>MMSETAPLPSASSALEDKAASAPVVGIIMGSQSDFETMRHADALLTELEIPHET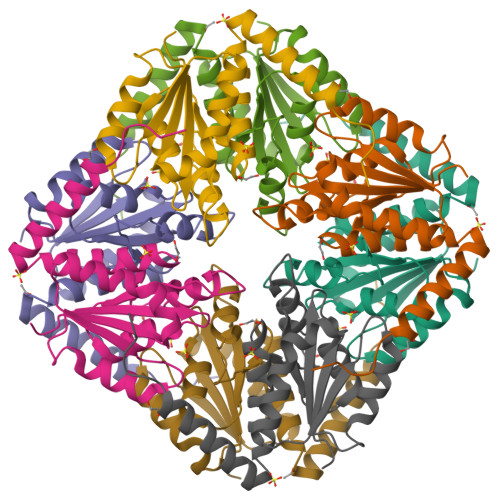LIVSAHRTPDRLADYARTAAERGLNVIIAGAGGAAHLPGMCAAWTRLPVLGVPVESRALKGMDSLLSIVQMPGGVPVGTLAIGASGAKNAALLAASILALFNPALAARLETFRALQTASVPNSPITEDK[2x]> MIRAVFFDSWGTLISVEGAYKVHFKIMEEVLGDYPLNPKTLLDEYEKLAREAFSNNAGKPYRPLRDILEEVMRKLAEKYGFKYPENLWEISLRMAQRYGELYPEVVEVLKSLKGKYHVGVILNRDTEPST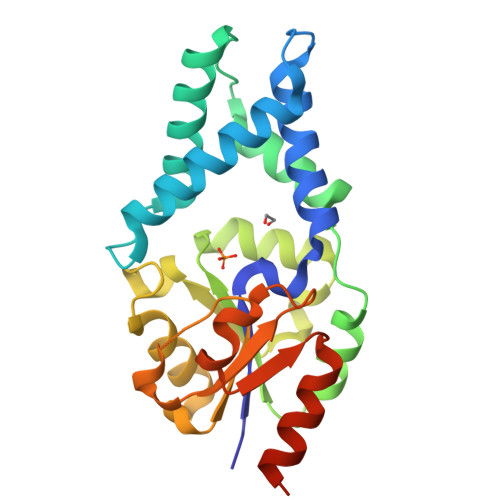AFLDALGIKDLFDSITTSEEAGFSKPHPRIFELALKKAGVKGEKAVCVGPNPVKDAGGSKNLGMTSILLDRKGEKREFWDKADFIVSDLREVIKIVDELNGQGSLEHHHHHH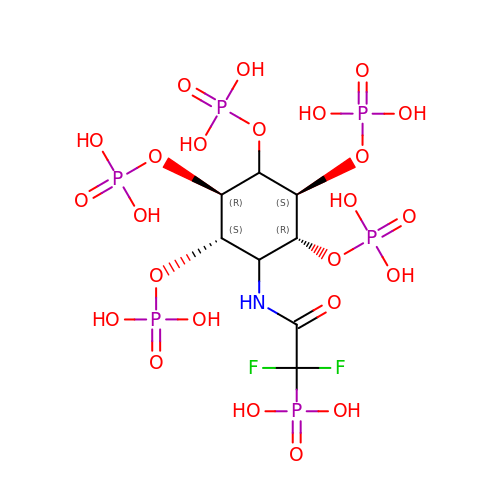(1,1-difluoro-2-oxo-2-{[(1s,2R,3S,4s,5R,6S)-2,3,4,5,6-pentakis(phosphonooxy)cyclohexyl]amino}ethyl)phosphonic acid | C8 H19 F2 N O24 P6 | XBHZOGSBYRIXJA-QWBQGLJISA-N> MRVCYFVLVPSVALAVIATESSETSGTIVHVFPLRDVADHRNDALINRALR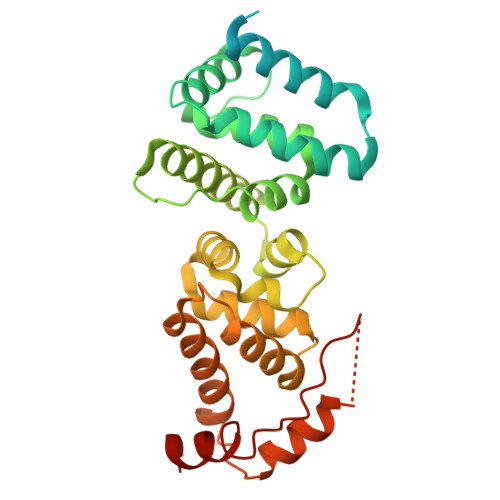AQTALDDDEERWPFGPSAVEALIETIDRHGRVSLNDEAKMKKVVRTWKKLIERDDLIGEIGKHYFEAPGPLHDTYDEALATRLVTTYSDRGVARAILHTRPSDPLSKKAGQAHRLEEAVASLWKGRGYTSDNVVSSIATGHDVDFFAPTAFTFLVKCVESEDDANNAIFEYFGSNPSRYFSAVLHAMEKPDADSRVLESSKKWMFQCYAQKQFPTPVFERTLAAYQSEDYAIRGARNHYEKLSLSQIEELVEEYSRIYSV>[2x]MGNKNTPLNSGKHPDLKIEVAIIGAGTSGLYTAYRLVTDKKFKAHDVQIFDMNNKLGGRLESVIMPGMNFWGELGGMRYLTSQQIVTTLIEGYPLSEKDPNKRTPVLKDKMTPVPFPMGDPSKLLMYLRKERFKQNAWNEAQKKGEKLPTRYYLNENDLGFSSDQLFNKIIYDVLMADPWVAETYGSKIIKGSSVYDY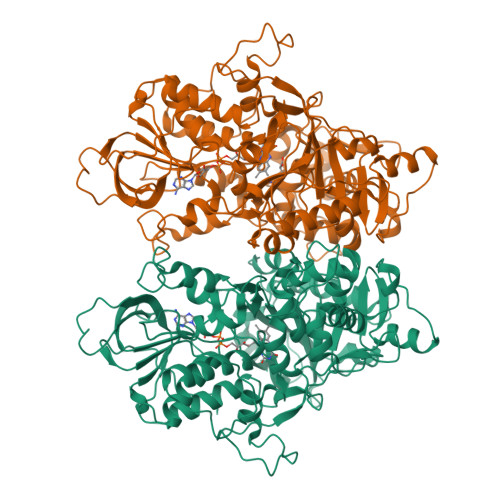SFKLTSRDWDDIKPKLVYNFPNSPYDQRKVNDIGFWNLIKDQVSQEGYEFLANAGGYYSNTINWNSAEAFPYMVGDFSAGTIYKTIEEGYDSIAYAVANSYMEHEGACIWSENKLLTFTKDHPLTNTHKYELTFLNLKTNTQWKVYANSIVLAMPRKSLELLDQNNFFFNINKNSVLNNNIRSVIMEPAFAILMGFEYPWWKELGIDSGHSITDLPMRQCYYFGTDPETNNSMLLGSYGDMETETFWKALSDDKVLFEVKAAKSASLRELHQLDDVQATKLMVGELMNQLRELHGDTVTIPEPYVTYFKDWTDEPFGAGYHAWKAGFSVENVMPYMRKPLTDEQIHICGEAYSDQQGWVEGAFCEAEKMLQEYFGLDRPYWLSPDYYLGWEHHHHHH> MTIDQKNTNIDPRFPHHHPRPQSFWEARAKALESLLIEKGHLSSDAIERVIKHYEHELGPMNGAKVVAKAWTDPAFKQRLLEDSETVLRELGYYGLQGEHIRVVENTDTVHNVVVCTLCSCYPWPLLGLPPSWYKEPAYRARVVKEPRQVLKEFGLDLPDSVEIRVWDSSSEIRFMVLPQRPEGTEGMTEEELAKLVTRDSMIGVAKIEPPKVTVG;> MNGIH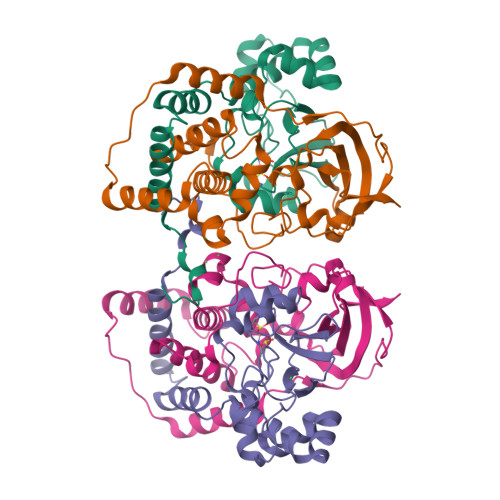DVGGMDGFGKVMYVKEEEDIYFTHDWERLAFGLVAGCMAQGLGMKAFDEFRIGIELMRPVDYLTSSYYGHWIATVAYNLVDTGVLDEKELDERTEVFLKKPDTKIPRREDPALVKLVEKALYDGLSPLREISASPRFKVGERIKTKNIHPTGHTRFPRYARDKYGVIDEVYGAHVFPDDAAHRKGENPQYLYRVRFEAEELWGYKQKDSVYIDLWESYMEPVSH>[2x]MKKALICIDYTNDFAAENGALTCGEPARQIE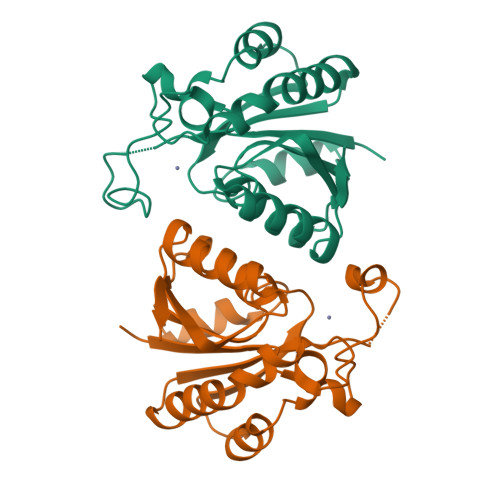DTIVSLTQAFIENGDYVVFAVDSHDADDDFHPETRLFPPHNINGTEGKELYGRLSPLYEKHKHAKNVNYMEKTRYSAFAGTDLELKLRERQITELHLAGLCTDICVLHTAVDAYNKGFQIVIHQNAVASFNPEGHEWALSHFKNSIGAQVAE> MSPPTASASVASSGSSPHMDRLLGDLKLLAAYDSAAGWQ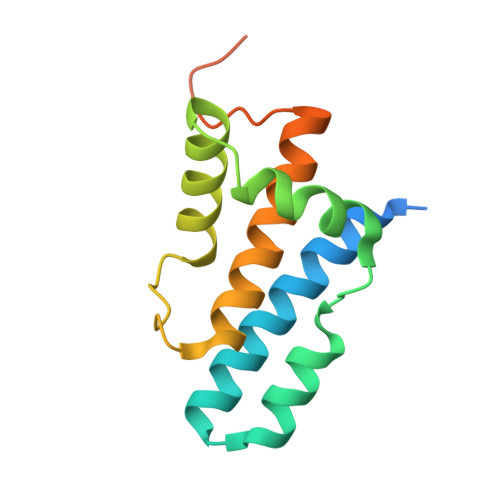EPKAMESAFQSLSWDDADVLKALPQYLNCRGEQKRRVDFAYAALCPRPVDEKDPKQTLMSLWMKARLFSYDQKHPFVLSPFAATDKSTSAGAMTAEKPF>[2x]GSHMASMKKKGSVVIVGRINLSGDTAYAQQTRGEEGCQETSQTGRDKNQVEGEVQIVSTATQTF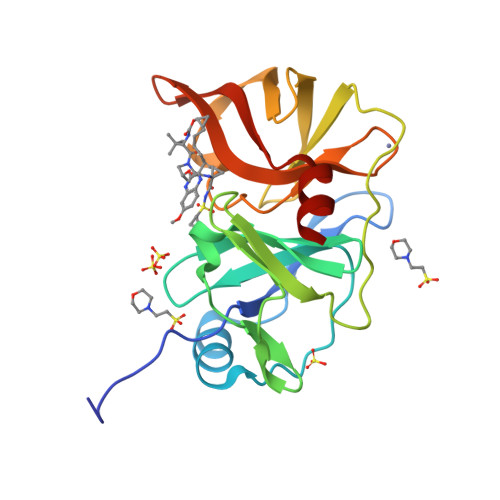LATSINGVLWTVYHGAGTRTIASPKGPVTQMYTNVDKDLVGWQAPQGSRSLTPCTCGSSDLYLVTRHADVIPVRRRGDSTGSLLSPRPLSYLKGSSGGPLLCPAGHAVGIFRAAVSTRGVAKAVQFIPVESLETTMRSP>[3x]GMKVTFLGAAVVLIEGKKNIII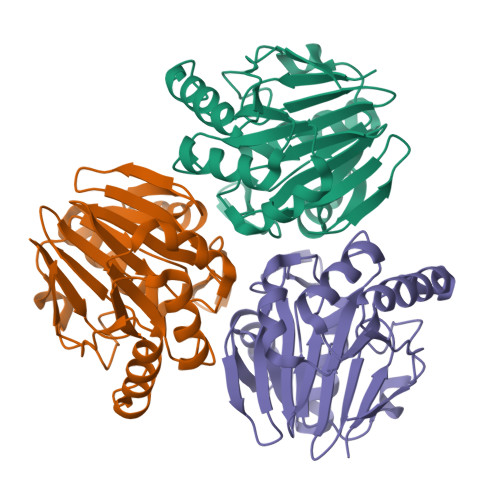DPFISGNPVCPVKLEGLPKIDYILVTHGHGDHLGDAVEIAKKNDATVISNYEICHYLGKKGVKTHAMHIGGSYLFDFGRVKMTPAVHGSGILDGDSMIYGGNPSGFLITIEGKKIYHAGDTGLTREMELLAEENVDVAFLPIGGNFVMDVEDAVRAAVMIKPKKVVPMHYGTWELIFADVELFKKKVEEKGVECVILEPGESLEL> SHVENDYIDNPSL;> GSLIGLMKDAFQPHHHHHHHLSPHPPGTVDKKMVEKCWKLMDKVVRLCQNPKLALKNSPPYILDLLPDTYQHLRTILSRYEGKMETLGE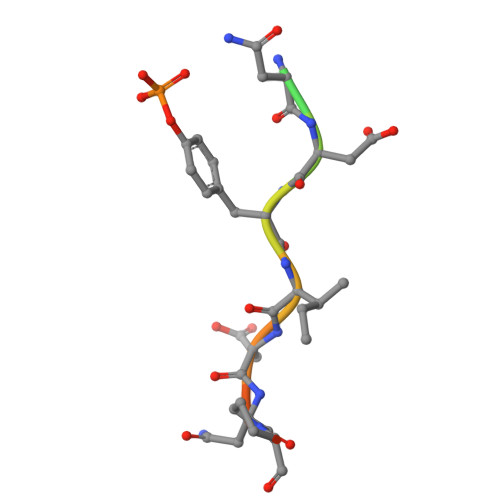NEYFRVFMENLMKKTKQTISLFKEGKERMYEENSQPRRNLTKLSLIFSHMLAELKGIFPSGLFQGDTFRITKADAAEFWRKAFGEKTIVPWKSFRQALHEVHPISSGLEAMALKSTIDLTCNDYISVFEFDIFTRLFQPWSSLLRNWNSLAVTHPGYMAFLTYDEVKARLQKFIHKPGSYIFRLSCTRLGQWAIGYVTADGNILQTIPHNKPLFQALIDGFREGFYLFPDGRNQNPDLTG> MHHHHHHNRQQIDALVKQMNVDTAKGPVD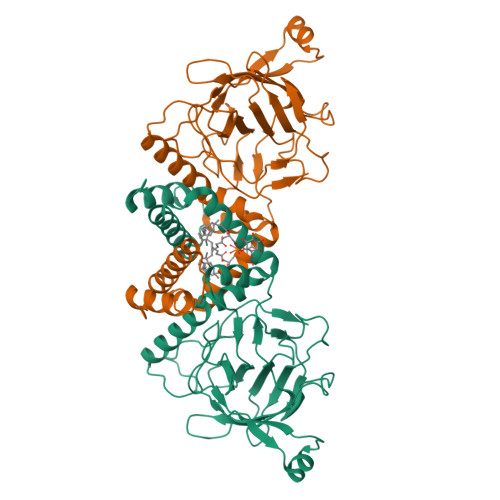ERIQQVVVRLLGDLFQAIEDLDIQPSEVWKGLEYLTDAGQANELGLLAAGLGLEHYLDLRADEADAKAGITGGTPRTIEGPLYVAGAPESVGFARMDDGSESDKVDTLIIEGTVTDTEGNIIEGAKVEVWHANSLGNYSFFDKSQSDFNLRRTILTDVNGKYVALTTMPVGYGCPPEGTTQALLNKLGRHGNRPSHVHYFVSAPGYRKLTTQFNIEGDEYLWDDFAFATRDGLVATATDVTDEAEIARRELDKPFKHITFNVELVKEAEAAPSSEVERRRASA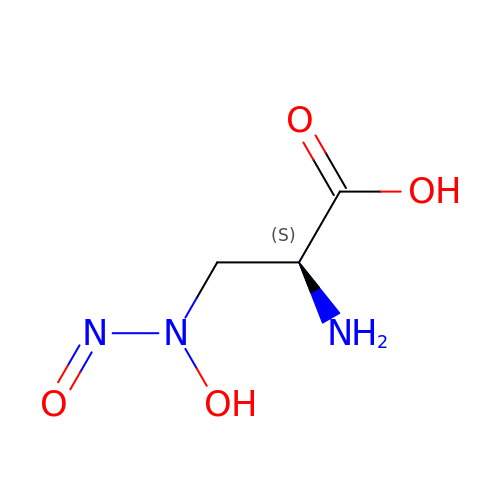3-[HYDROXY(NITROSO)AMINO]-L-ALANINE | C3 H7 N3 O4 | MLFKVJCWGUZWNV-REOHCLBHSA-N>SMGNMCMVMFGYDMIHITVFQPDKSRSEYCDEIPATGRTIMAFDIENPAFRDLPLELR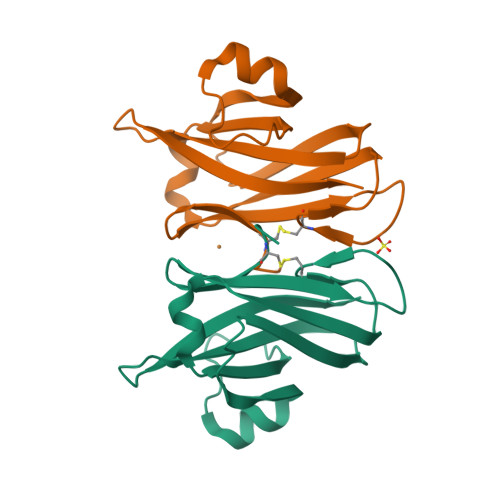IIRDPLTPVLPTGEKELDALTELHLPAKKYSKGTFSVEHNFANNGHYIGLVTLTRESGQQETAQFKFMVG[2x]> GGUCCGUUGAAGACUGCAGGAGAGUGGUUGUUAACCAGAUUUUAAC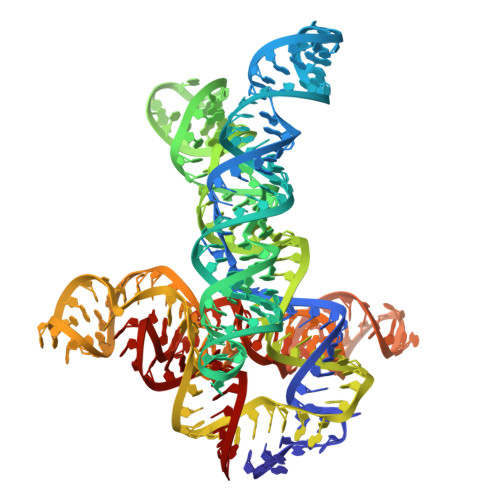AUCUGAGCCAAAUAACCCGCCGAAGAAGUAAAUCUUUCAGGUGCAUUAUUCUUAGCCAUAUAUUGGCAACGAAUAAGCGAGGACUGUAGUUGGAGGAACCUCUGGAGAGAACCGUUUAAUCGGUCGCCGAAGGAGCAAGCUCUGCGCAUAUGCAGAGUGAAACUCUCAGGCAAAAGGACAGAGGA>GSMAELKQEWINTAIEALDKAYVPYSHFPVGACLVTESGKIYQGINIENASFGLTNCAERTAFFKAVSEGERSFTHLVVAGHTPDPISPCGACRQVMAEFCAPDMPVTLVGDNGVTKATTVRELLPYAFTEKDL[2x]

As a zinc ion–dependent enzyme, CDA participates in the pyrimidine salvage pathway by converting cytidine and deoxycytidine into uridine and deoxyuridine. Bacteria extensively exhibit two forms of CDA: a long form and a short one. The former harbors two tandem CDA domains typically structured in a dimer assembly (homodimeric CDA or D-CDA), while the latter possesses a single catalytic domain arranged in a tetramer assembly (termed homotetrameric CDA or T-CDA). The CDA derived from E. faecium (EfCDA) belongs to the T-CDA form. EfCDA showed the ability to convert gemcitabine to its metabolite 2′,2′-difluorodeoxyuridine.

The investigation of the interaction between EfCDA and gemcitabine involved the co-crystallization of EfCDA and gemcitabine. Due to the similar molecular structure shared by gemcitabine and dFdU, distinguishing between these two molecules based solely on the electron density map pattern posed a challenge. However, considering the catalytic activity of EfCDA, it was anticipated that gemcitabine would be rapidly converted to dFdU. As a result, the molecule identified in the co-crystallized crystals was determined to be dFdU. The dFdU molecule, situated within a pocket delineated by molecules A, C, and D, exhibited interaction interface areas measuring 176.4 Å2, 70.8 Å2, and 61.0 Å2, respectively, suggesting that these individual molecules all contribute to the binding of dFdU. Additionally, the O4 of the dFdU molecule, working in unison with C55, C88, and C91, demonstrated chelation with Zn2+. Hydrogen bond formation was observed between E57 and O4 and N3 of dFdU. The ribose ring of dFdU participates in the creation of multiple hydrogen bond interactions, wherein the O5′ forms hydrogen bonds with the amide group of A48 and F50, respectively, and the O3′ interacts with the side chains of N44 and E46 via hydrogen bonds. Notably, the two fluorine atoms of dFdU establish hydrogen bonds with the hydroxyl group of S49 and the amide nitrogen of G51 via a water molecule. Furthermore, the dFdU molecules were discovered to interact with F26, V28, T53, F127, and L132 through hydrophobic interactions.> MIKLVFRYSPTKTVDGFNELAFGLGDGLPWGRVKKDLQNFKARTEGTIMIMGAKTFQSLPTLLPGRSHIVVCDLARDYPVTKDGDLAHFYITWEQYITY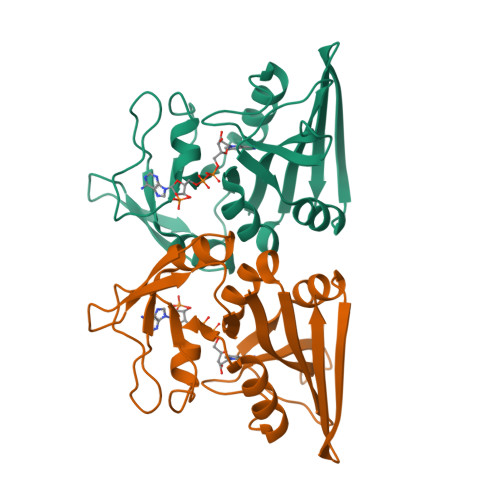ISGGEIQVSSPNAPFETMLDQNSKVSVIGGPALLYAALPYADEVVVSRIVKRHRVNSTVQLDASFLDDISKREMVETHWYKIDEVTTLTESVYK>[2x]MEPGPTAAQRRCSLPPWLPLGLLLWSGLALGALPFGSSPHRVFHDLLSEQQLLEVEDLSLSLLQGGGLGPLSLPPDLPDLDPECRELLLDFANSSAELTGCLVRSARPVRLCQTCYPLFQQVVSKMDNISRAAGNTSESQSCARSLLMADRMQIVVILSEFFNTTWQEANCANCLTNNSEELSNSTVYFLNLFNHTLTCFEHNLQGNAHSLLQTKNYSEVCKNCREAYKTLSSLYSEMQKMNELENKAEPGTHLCIDVEDAMNITRKLWSRTFNCSVPCSDTVPVIAVSVFILFLPVVFYLSSFLHSEQKKRKLILPKRLKSSTSFANIQENSNLEHHHHHHHH;>M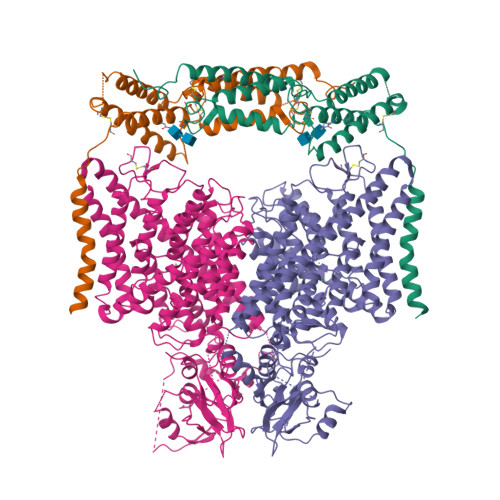ASDYKDDDDKASDEVDAGTMANVSKKVSWSGRDRDDEEAAPLLRRTARPGGGTPLLNGAGPGAARQSPRSALFRVGHMSSVELDDELLDPDMDPPHPFPKEIPHNEKLLSLKYESLDYDNSENQLFLEEERRINHTAFRTVEIKRWVICALIGILTGLVACFIDIVVENLAGLKYRVIKGNIDKFTEKGGLSFSLLLWATLNAAFVLVGSVIVAFIEPVAAGSGIPQIKCFLNGVKIPHVVRLKTLVIKVSGVILSVVGGLAVGKEGPMIHSGSVIAAGISQGRSTSLKRDFKIFEYFRRDTEKRDFVSAGAAAGVSAAFGAPVGGVLFSLEEGASFWNQFLTWRIFFASMISTFTLNFVLSIYHGNMWDLSSPGLINFGRFDSEKMAYTIHEIPVFIAMGVVGGVLGAVFNALNYWLTMFRIRYIHRPCLQVIEAVLVAAVTATVAFVLIYSSRDCQPLQGGSMSYPLQLFCADGEYNSMAAAFFNTPEKSVVSLFHDPPGSYNPLTLGLFTLVYFFLACWTYGLTVSAGVFIPSLLIGAAWGRLFGISLSYLTGAAIWADPGKYALMGAAAQLGGIVRMTLSLTVIMMEATSNVTYGFPIMLVLMTAKIVGDVFIEGLYDMHIQLQSVPFLHWEAPVTSHSLTAREVMSTPVTCLRRREKVGVIVDVLSDTASNHNGFPVVEHADDTQPARLQGLILRSQLIVLLKHKVFVERSNLGLVQRRLRLKDFRDAYPRFPPIQSIHVSQDERECTMDLSEFMNPSPYTVPQEASLPRVFKLFRALGLRHLVVVDNRNQVVGLVTRKDLARYRLGKRGLEELSLAQT[2x]6-(propylsulfanyl)-1,5-dihydro-4H-pyrazolo[3,4-d]pyrimidin-4-one 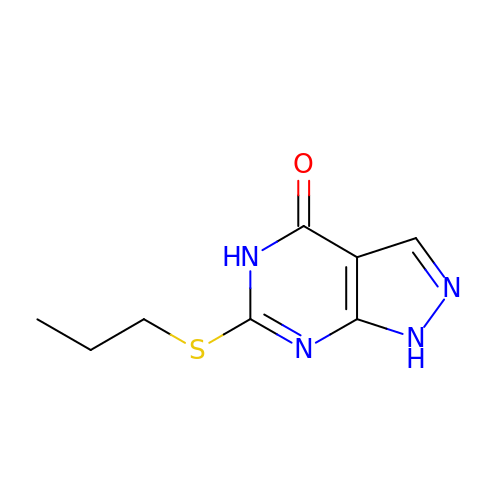| C8 H10 N4 O S | CNXWMVZWQIUZRK-UHFFFAOYSA-N2,5-bis(2-hydroxyethyl)-1,3-oxazole-4-carboxylic acid | C8 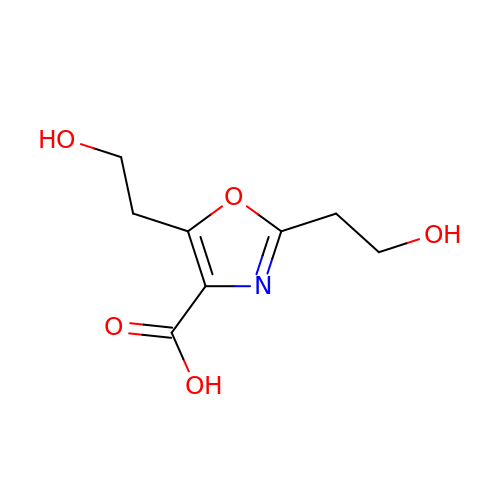H11 N O5 | PLUGCRBIUHQSBZ-UHFFFAOYSA-N> MRGSHHHHHHGRSLNPLSTPQFDSTDETPASYNLAVRRAAPAVVNVYNRGLNTNSHNQLEIRTLGSGVIMDQRGYIITNKHVINDADQIIVALQ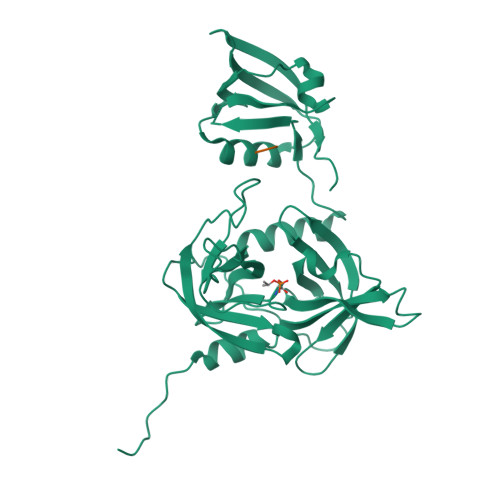DGRVFEALLVGSDSLTDLAVLKINATGGLPTIPINARRVPHIGDVVLAIGNPYNLGQTITQGIISATGRIGLNPTGRQNFLQTDASINPGNSGGALVNSLGELMGINTLSFDKSNDGETPEGIGFAIPFQLATKIMDKLIRDGRVIRGYIGIGGREIAPLHAQGGGIDQLQGIVVNEVSPDGPAANAGIQVNDLIISVDNKPAISALETMAQVAEIRPGSVIPVVVMRDDKQLTLQVTIQEYPATN;> YQF>MGSSHHHHHHSSGENLYFQGHMASMESASLDQSAALLVKELTEHIDDSNGLGFMSPAIYDTAWVSMIKKTDNDQTFWLFPKSFHYILENQLENGGWVTYASEIDGILNTSASLLSLKRHFDLPLQISTESQTSMENRIRKATDALRVLLRTWDVDATLHVGFEILVPALLDYLQVEGLTFDFPGRDKLFQIRDQKLSRFKPEFIYAPFQTTALHSLEAFIGLIDFDRVQHHKVRGSFMASPSSTAAVLMNATEWDIDCEEYIRHVIEHASGKASGGVPSAFPSTIFEITWTLSTLLKAGFNLSSNDSSNVQKACSYLLGVLTAEKGAIGFVPSVCADADDTAKTILVLSLLRENVLPDGMLKAFEVENHFKTYPLERDPSFSANCNVLLALLHLENPSQYTLQIEKATRFLYTHFRESNLNVRDKWNLSPFYSWMLMAQAIARLDELCKGSQLKNLHDHVESDLIPLLQEMTVSVMHQQNKDGSWGTKLSKEETAYAVLMLTYAVSFEALVGPRRQIRNAIEEGCLFLRSGKDATSERLWVEKVTYESQMLSRAYTLAALKNALDVLKKDDMKIAFIGNSVNESFTEIEVVNGKNVTEPSSNTYDLKEVKMD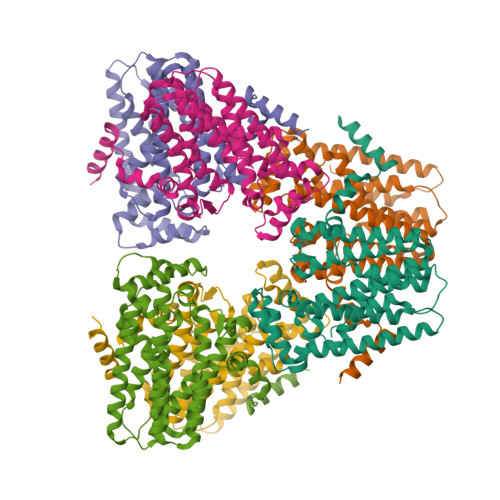KAEFTPPDTPPRSKSTSVDPIEEAICAHENRGAISDHTSRAIDLCRNPPLWGTDQEQTLLGPFEYLESIPGKNIRSQFIEAFNTWLQIPQDHLQIVGKVISMLHTASLLVDDIEDNSLLRRGQPVAHSIFGTAQTFNSGNYVYFLALQEVQKLNSPRAISIFVDALTQLHRGQGMDVFWRDSLICPTEEEYLDMVANKTGALFCLAIELLQIKSTVQLDFLPLVRLLGIIFQICDDYLNLKSTNYTQKKGLCEDITEGKFSFPIIHSIRTKPGNRQLINVLRQKSKEDDVKRFALAYMESTQSFDYTRDFVKILNGEALRMIEDLEQQGLHRNIEIRNILARMSLEQ[6x]> MGYYDDDAHGHVEADAAPRATTGTGTGSASQTVTIPCHHIRLGDILILQGRPCQVIRISTSAATGQHRYLGVDLFTKQLHEESSFVSNPAPSVVVQTMLGPVFKQYRVLDMQDGSIVAMTETGDVKQN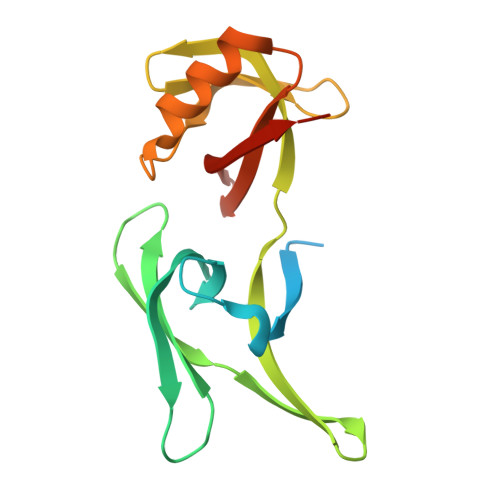LPVIDQSSLWNRLQKAFESGRGSVRVLVVSDHGREMAVDMKVVHGSRLA> MDNVPTFPRDYEGPFDVTEGQPGPRVWTFLAHDRDSGPNGQVEYSVVDGDPLGEFVISPVEGVLRVRKDVELDRETIAFYNLTICARDRGVPPLSSTMLVGIRVLDINDNDPVLLNLPMNVTISENS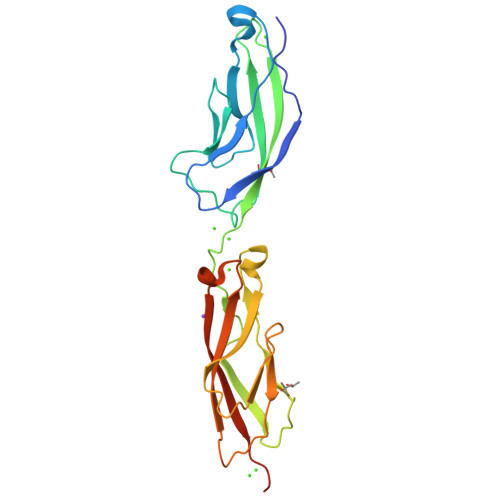PVSSFVAHVLASDADSGCNALLTFNITAGNRERAFFINATTGIVTVNRPLDRERIPEYRLTVSVKDNPENPRIARKDFDLLLVSLADENDLEHHHHHH8-[[(3R,4R)-3-[[1,1-bis(oxidanylidene)thian-4-yl]methoxy]piperidin-4-yl]amino]-3-methyl-1H-1,7-naphthyridin-2-one | C20 H28 N4 O4 S | 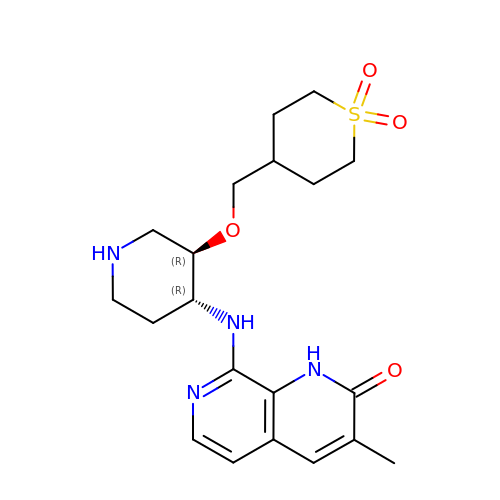IMRGYBMGTASFSC-IAGOWNOFSA-N>[2x]MSLKSIEVVAAVIRLGEKYLCVQRGQTKFSYTSFRYEFPGGKVEEGESLQEALQREIMEEMDYVIEVGEKLLT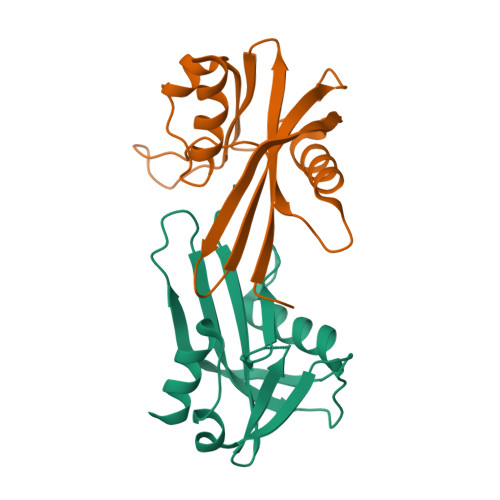VHHTYPDFEITMHAFLCHPVGQRYVLKEHIAAQWLSTREMAILDWAEADKPIVRKISEQEGHHHHHH> GRCTKS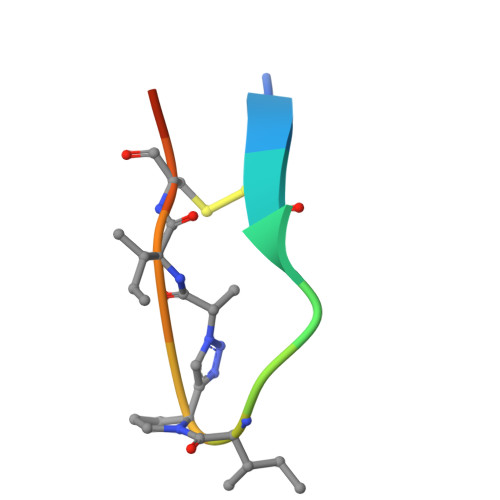IXICFPD>[2x]MGSSHHHHHHSSGENLYFQGHMSSTFEPATDSPLPVPGVQYFLQHVQSGKYVHPHGGSDMPGNDTALVLHHGFDEKRDALRWVFVNDAENKHQLKHYSSGKFVHPKGGKVGKEATLVVHSSPGRPETMIEMVQEDGRTYLRHTDSDYYVHPH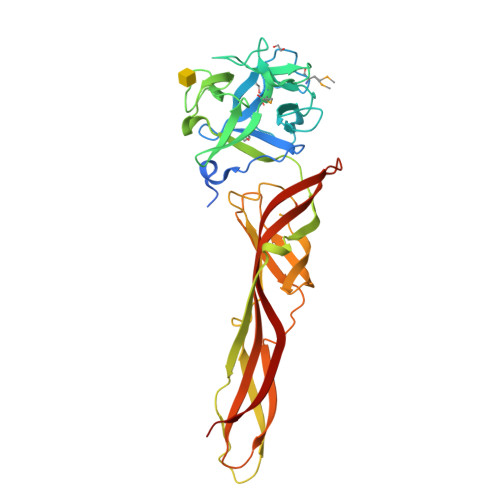GGSPNPGDNTRLVYYSGYRPSLAFLAIPAETLFVDRIEIHQAQALESINTITSLSDEHRNDTDQPVQTSISVALEESLQDSAQLSFERCFGLKVGSEFEVGLPLVGKTKVSVQFSGSWKSSTIKGEVRTSAVKVQINEHVTIPPGKCVQIRIDTRRCTKTAPATMYLRTASGIEVQRETTVTSTYHYDQEVHVVPVTN>MATEPKAGRPSDYMPEVADDICSLL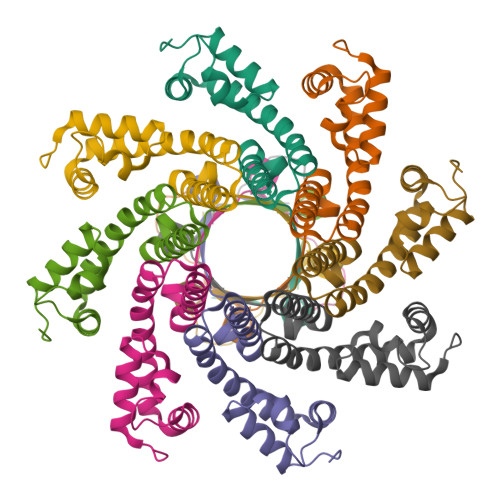SSGESLLKVCKRPGMPDKSTVFRWLAKHEDFRDKYAKATEARADSIFEEIFEIADNAIPDAAEVAKARLRVDTRKWALARMNPRKYGDKVTNELVGKDGGAIQIETSPMSTLFGK[2x]>GSHMSQEEKLPKILIVEDDERLARLTQEYLIRNGLEVGVETDGNRAIRRIISEQPDLVVLDVMLPGADGLTVCREVRPHYH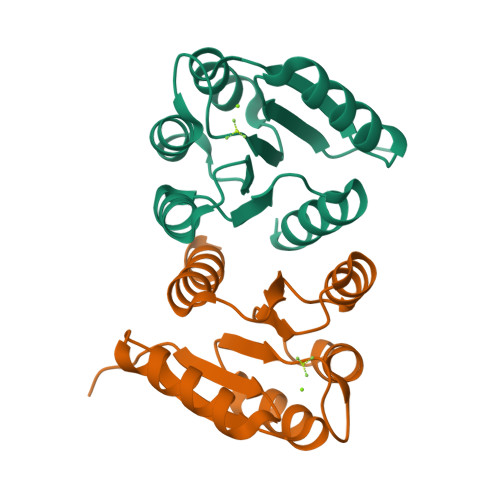QPILMLTARTEDMDQVLGLEMGADDYVAKPVQPRVLLARIRALLRRTDKTVE[2x]(6R)-4-hydroxy-6-methyl-3-(propan-2-yl)cyclohexa-2,4-dien-1-one 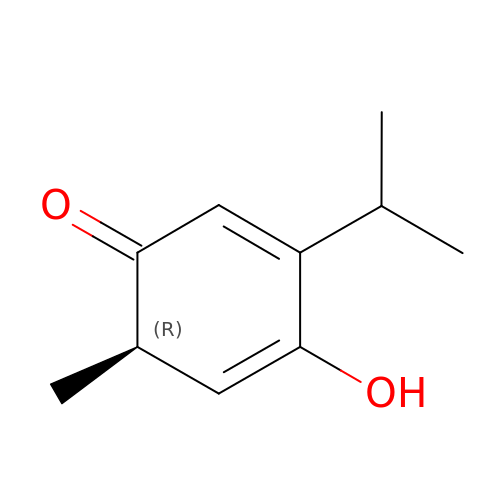| C10 H14 O2 | QZGDYXFNICWHLG-UHFFFAOYSA-N N-{5-[(7-{[(2S)-2-HYDROXY-3-PIPERIDIN-1-YLPROPYL]OXY}-6-METHOXYQUINAZOLIN-4-YL)AMINO]PYRIMIDIN-2-YL}BENZAMIDE 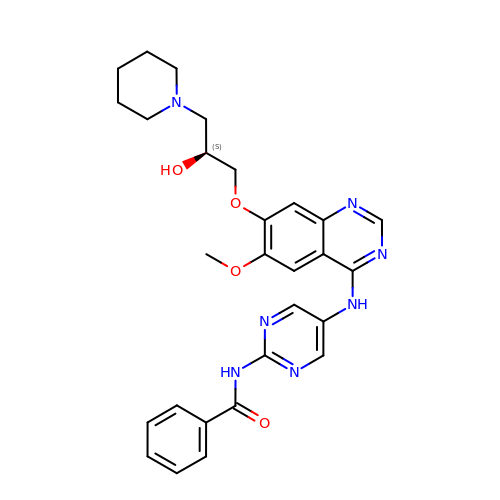| C28 H31 N7 O4 | WHHFZOIADLFZRX-NRFANRHFSA-N>MGATSWLDGSGQIHLRIYSLQQSNGKLLERCWDSNKWYDGALTN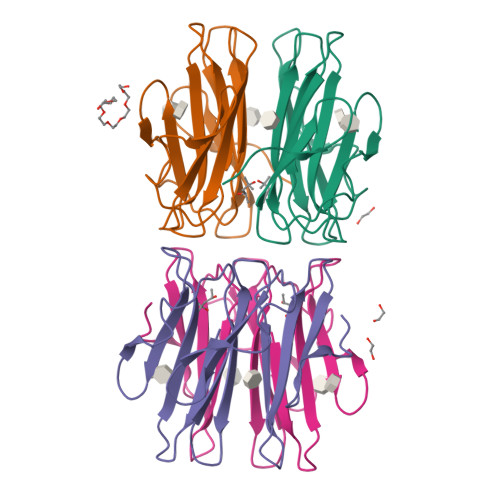QFSAISGAGATSWLDSSGQIHIRVYAIGTDGKIIELCWDKDKWYSGALTGQFYGASTPDATSWLDKNGQIHIRVYAYNQDNVQKEYCWDGSKWYVGAYTE[6x]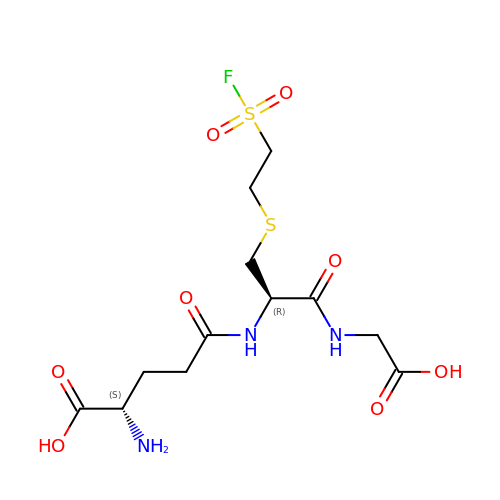(2S)-2-azanyl-5-[[(2R)-3-(2-fluorosulfonylethylsulfanyl)-1-(2-hydroxy-2-oxoethylamino)-1-oxidanylidene-propan-2-yl]amino]-5-oxidanylidene-pentanoic acid | C12 H20 F N3 O8 S2 | ICNGQPVIPUWGEA-YUMQZZPRSA-N>AAALAAAAPRTVYAFSARPLAGGEPFNLSSLRGKVLLIENVASLUGTTVRDYTQMNDLQRRLGPRGLVVLGFPCNQFGHQENAKNEEILNCLKYVRPGGGFEPNFMLFEKCEVNGEKAHPLFAFLREVLPTPSDDATALMTDPKFITWSPVCRNDVSWNFEKFLVGPDGVPVR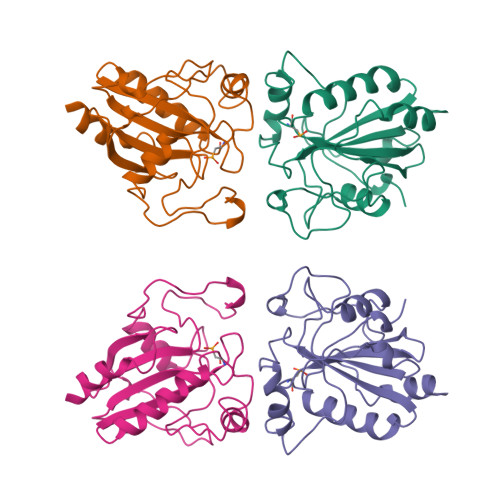RYSRRFLTIDIEPDIETLLSQGASA[2x]>[2x]MLVKGNEILLKAHKEGYGVGAFNFVNFEMLNAIFEAGNEENSPLFIQASEGAIKYMGID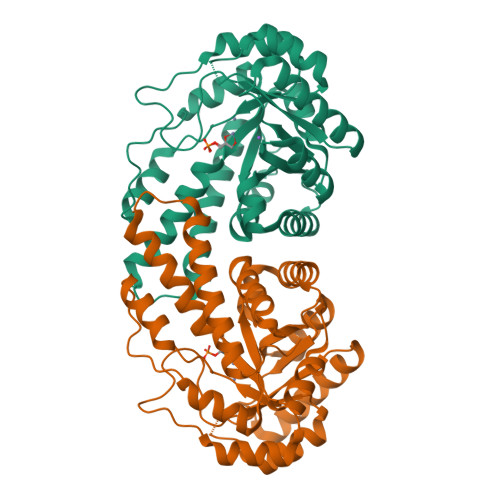MAVGMVKIMCERYPHIPVALHLDHGTTFESCEKAVKAGFTSVMIDASHHAFEENLELTSKVVKMAHNAGVSVEAELGRLMGIADNISVDEKDAVLVNPKEAEQFVKESQVDYLAPAIGTSHGAFKFKGEPKLDFERLQEVKRLTNIPLVLHGASAIPDNVRKSYLDAGGDLKGSKGVPFEFLQESVKGGINKVNTDTDLRIAFIAEVRKVANEDKSQFDLRKFFSPAQLALKNVVKERMKLLGSANKI>MAVPPTYADLGKSARDVFTKGYGFGLIKLDLKTKSENGLEFTSSGSANTETTKVTGSLETKYRWTEYGLTFTEKWNTDNTLGTEITVEDQLARGLKLTFDSSFSPNTGKKNAKIKTGYKREHINLGCDMDFDIAGPSIRGALVLGYEGWLAGYQMNFETAKSRVTQSNFAVGYKTDEFQLHT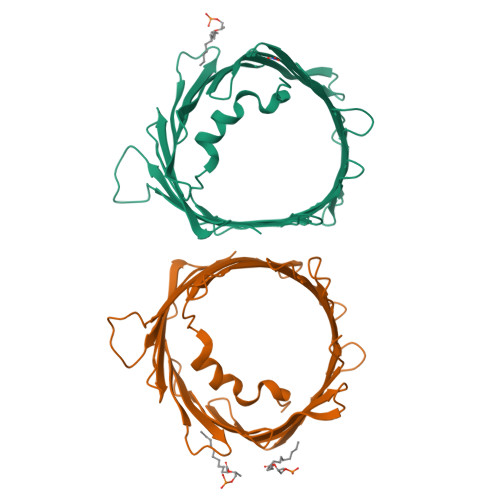NVNDGTEFGGSIYQKVNKKLETAVNLAWTAGNSNTRFGIAAKYQIDPDACFSAKVNNSSLIGLGYTQTLKPGIKLTLSALLDGKNVNAGGHKLGLGLEFQALEHHHHHH[2x]>[2x]MNTVPFTSAPIEVTIGIDQYSFNVKENQPFHGIKDIPIGHVHVIHFQHADNSSMRYGYWFDCRMGNFYIQYDPKDGLYKMMEERDGAKFENIVHNFKERQMMVSYPKIDEDDTWYNLTEFVQMDKIRKIVRKDENQFSYVDSSMTTVQENELSSSSSDPAHSLNYTVINFKSREAIRPGHEMEDFLDKSYYLNTVMLQGIFKNSSNYFGELQFAFLNAMFFGNYGSSLQWH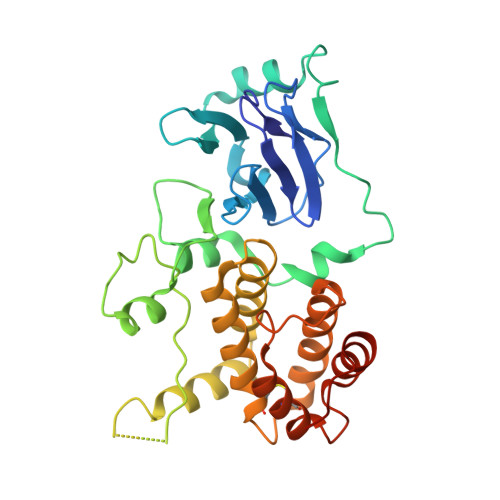AMIELICSEATVPKHMLDKLDEILYYQIKTLPEQYSDILLNERVWNICLYSSFQKNSLHNTEKIMENKYPELLGLEHHHHHH3-AMINOPYRIDINE-ADENINE DINUCLEOTIDE PHOSPHATE | C20 H29 N7 O16 P3 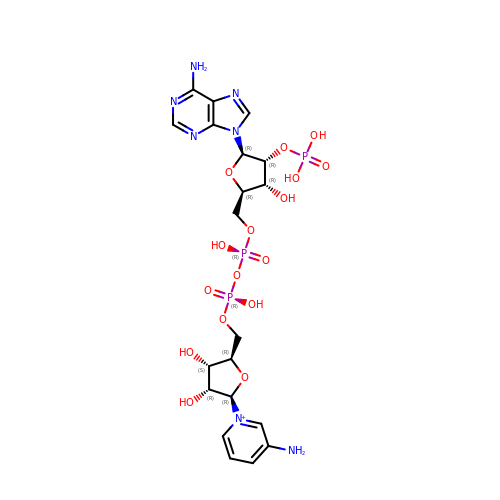| JRGQEVHOKKZPIX-HISDBWNOSA-O> TEATAGTVTVNAITSDDTIDGIELGQTISISGKAVGGDISVGDVVKMTINNTEYSTTVKAGGIWMIAGVLGSDLAADSEFDVVVTSSDAAGNKVQSIGTSTHSVDLSAEANFSLAEGQQHVLTNLPEGFGFPDGTTEVVTNFGGTITLGDDGEYRYDAPVRDHGDAVSDKDSVTVTLED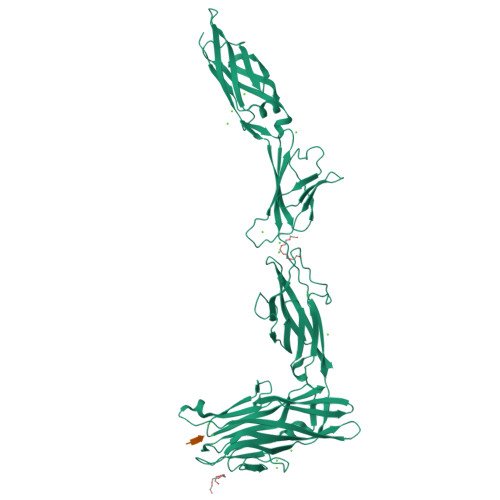GRTFTVNLDIQDSAPVAVDDQDSIVVQHEEFEVSEIAASWVSYTHGESVTTFDGTSDLGGVDNDSAKDQIRWGNPAESKQSGYGFIDNDSNLEGRFDLNQDISVGTFTHYNYPVYSGGAITSAEMSVEFSVLDHLGVSTPVTLTVNFDHNETPNTNDVNASRDIVTVQNTHVTFERDGDIYTVQIVGFREVGNPDGEVVTSIYTNENAATSYELVVRVVEGDGYSLPSTEGNIFDDNGLGADSLGADGSVTVVGVAVGAIVSSNESVGHSIEGQYGNLVLNSDGSYVYDVTASVSDIPAGATESFAYLIQDQDGSTSSANLSINVGTN;> DSD> GPPGPPGPPGPPGPAGFPGPPG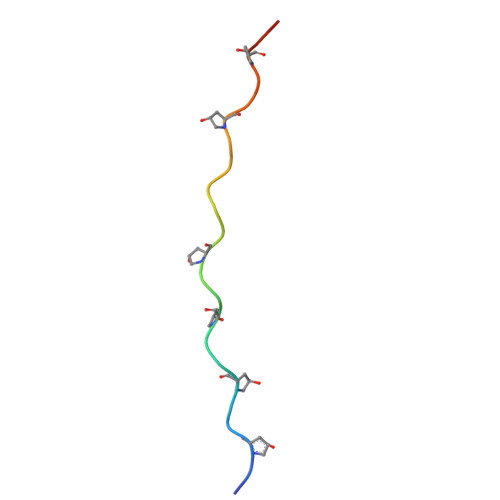PPG> VHFHPFGGVNFYEMDWSLKGDLWAHDPVIAKEGSRWYVFHTGSGIQIKTSEDGVHWENMGWVFPSLPDWYKQYVPEKDEDHLWAPDICFYNGIYYLYYSVSTFGKNTSVIGLATNQTLDPRDPDYEWKDMGPVIHSTASDNYNAIDPNVVFDQEGQPWLSFGSFWSGIQLIQLDTETMKPAAQAELLTIASRGEEPNAIAAPFIVCRNGYYYLFVSFDFCCRGIESTYKIAVGRSKDITGPYVDKNGVSMMQGGGTILDEGNDRWIGPGHCAVYFSGVSAILVNHAYDALKNG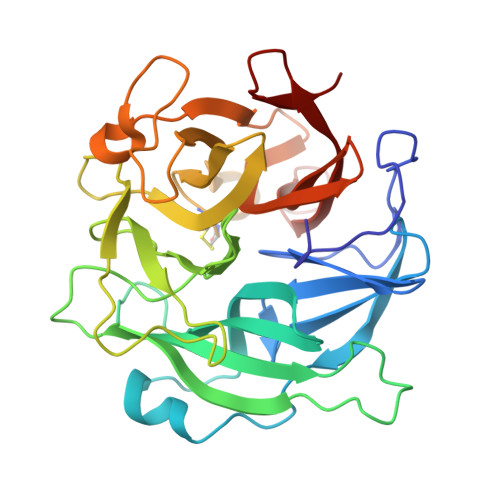EPTLQIRPLYWDDEGWPYLSV>MPVDKNLRDLEPGIHTDLEGRLTYGGYLRLDQLLSAQQPLSEPAHHDEMLFIIQHQTSELWLKLLAHELRAAIVHLQRDEVWQCRKVLARSKQVLRQLTEQWSVLETLTPSEYMGFRDVLGPSSGFQSLQYRYIEFLLGNKNPQMLQVFAYDPAGQARLREVLEAPSLYEEFLRYLARFG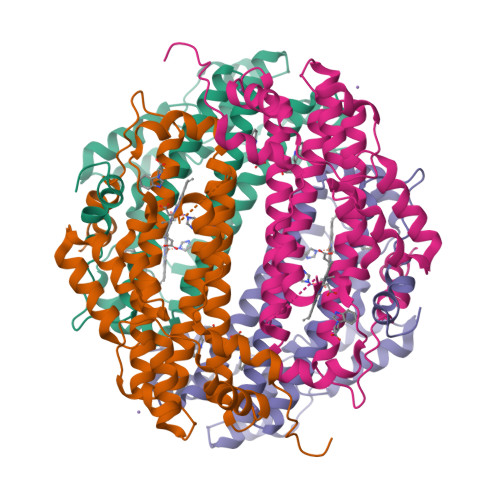HAIPQQYQARDWTAAHVADDTLRPVFERIYENTDRYWREYSLCEDLVDVETQFQLWRFRHMRTVMRVIGFKRGTGGSSGVGFLQQALALTFFPELFDVRTSVGVDNRPPQGSADAGKRLEHHHHHH[2x]N-[(E)-3-[(2R,3S,4R,5R)-3,4-dihydroxy-5-[4-(trifluoromethyl)imidazol-1-yl]oxolan-2-yl]prop-2-enyl]-2,3-dihydroxy-5-nitro-benzamide | C18 H17 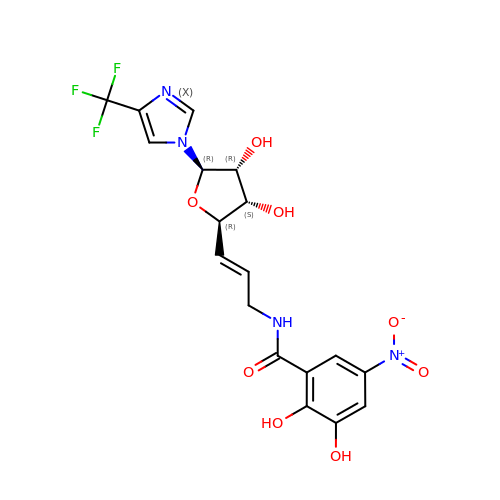F3 N4 O8 | VZQNYKXXPHSQLJ-LWULHLCXSA-N> QGHMTIHDRKEFAKFEEERARAKWDTANNPLYKEAMVALSLKISIGNVVKTMQFEPSTMVYDACRMIRERIPEALAGPPNDFGLFLSDDDPKKGIWLEAGKALDYYMLRNGDTMEYRKKQRPLKIRMLDGTVKTIMVDDSKTVTDMLMTICARIGITNHDEYSLVRELMEEKKDELNWLDHGRTLREQGVEEHETLLLRRKFFYSDQNVDSRDPVQLNLLYVQARDDILNGSHPVSFDKACEFAG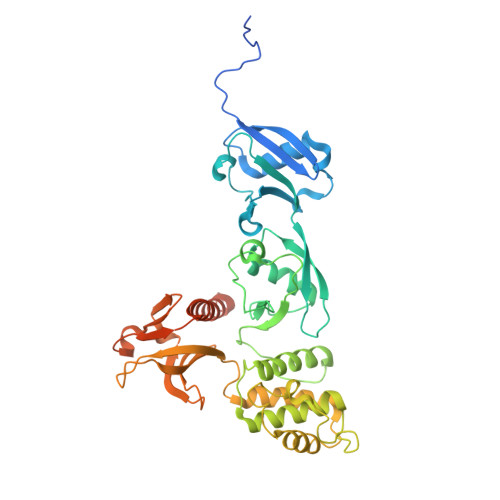FQCQIQFGPHNEQKHKAGFLDLKDFLPKEYVKQKGERKIFQAHKNCGQMSEIEAKVRYVKLARSLKTYGVSFFLVKEKMKGKNKLVPRLLGITKECVMRVDEKTKEVIQEWSLTNIKRWAASPKSFTLDFGDYQDGYYSVQTTEGEQIAQLIAGYIDIILKKKKSKDHFGLEGDEESTMLEDSVSPKKST>GPGSMAEHCPTPHNGAKYGEIAETVLMAGDPLRVKLLADTYLTDVVQYNSVRGAVGYTGYYKGVKLSVQAHGMGMPSIGIYAYELFNFYGVKRIIRIGSAGAFDESLKLGDIVIGMGACYDSNFERQYDIPGKYSCIADFQ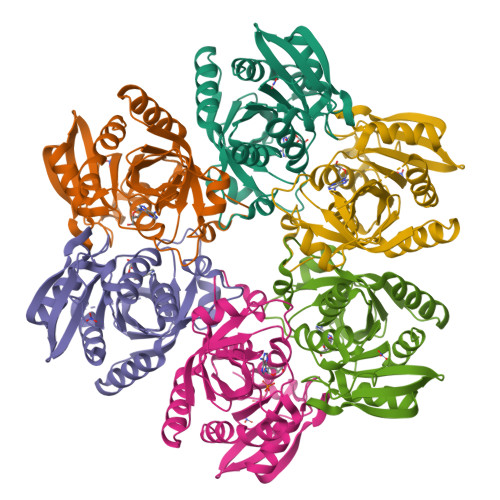LCREAVDAAEKLGYRYKVGNIYSANYFYDDGDHSGAWKKMGVLAVEMEAAALYMIAARARKQALCMLTISDLCYGSGEKMTAEERRTKFTQMMEVALSLAK[6x]Like other tailed, double-stranded (ds) DNA bacteriophages (order Caudovirales), the 80α capsid protein (CP, 324 residues) is first assembled into an empty procapsid, requiring a scaffolding protein (SP, 206 residues), which acts as a chaperone for the assembly process. The CP models show the expected HK97-like fold common to the Caudovirales, divided into A- and P-domains, with an extended E-loop and an N-arm that folds along the inside of the P-domain. Many SaPIs also cause the redirection of the helper phage assembly pathway to form capsids that are smaller than those normally formed by the phage and are therefore unable to package complete phage genomes. For SaPI1, we previously demonstrated that this size redirection depended on the SaPI1-encoded proteins CpmA and CpmB, leading to the formation of a 45 nm diameter capsid with T = 4 icosahedral symmetry.

There are seven CP subunits (A–G) in the asymmetric unit in the T = 7 80α procapsid structure, which are organized into A5 pentamers and BCDEFG hexamers. The 80α procapsid map had a density next to N-arm helix α1 that was identified as the 16 C-terminal residues of SP, which were built de novo as an 11-residue amphipathic α-helix followed by a 5-residue ‘hook’. The lower density of this feature is indicative of low occupancy, consistent with the previously estimated CP:SP molar ratio of 2:1. The hook includes the conserved RIIK motif that was previously hypothesized to interact with CP. The RIIK motif points into the hydrophobic cleft between the A and P domains, where R202, I203 and I204 make numerous contacts with the CP. In the preceding α-helix, L194, I197, A198 and K201 make contacts predominantly with the N-arm α-helix of CP. In subunits C and F only, residues Q192, R199 and N206 contact the adjacent CP subunits (B and E, respectively), presumably reflecting the hexamer skew that shifts these subunits relative to each other. In the 80α procapsid, the C-terminal 21 residues of SP form a ‘helix-and-hook’ motif that interacts extensively with the CP, especially with the N-arm. The rest of the SP was not resolved in the high-resolution map, suggesting that it is disordered and/or not organized with icosahedral symmetry. In the absence of CpmB, the less curved shell allows the incorporation of additional hexamers before requiring a pentamer, resulting in the T = 7 shell.

>[7x]MEQTQKLKLNLQHFASNNVKPQVFNPDNVMMHEKKDGTLMNEFTTPILQEVMENSKIMQLGKYEPMEGTEKKFTFWADKPGAYWVGEGQKIETSKATWVNATMRAFKLGVILPVTKEFLNYTYSQFFEEMKPMIAEAFYKKFDEAGILNQGNNPFGKSIAQSIEKTNKVIKGDFTQDNIIDLEALLEDDELEANAFISKTQNRSLLRKIVDPETKERIYDRNSDSLDGLPVVNLKSSNLKRGELITGDFDKLIYGIPQLIEYKIDETAQLSTVKNEDGTPVNLFEQDMVALRATMHVALHIADDKAFAKLVPADKRTDSVPGEV;>MEENKLKFNLQFFADQSDDPDEPGGDGKKGNPDKKENDEGTEITFTPEQQKKVDEILERRVAHEKKKADEYAKEKAAEAAKEAAKLAKMNKDQKDEYEREQMEKELEQLRSEKQLNEMRSEARKMLSEAEVDSSDEVVNLVVTDTAEQTKSNVEAFSNAVKKAVNEAVKVNARQSPLTGGDSFNHSTKNKPQNLAEIARQKRIIKN[7x]>[2x]WGNLGHETVAYIAQSFVASSTESFCQNILGDDSTSYLANVATWADTYKYTDAGEFSKPYHFIDAQDNPPQSCGVDYDRDCGSAGCSISAIQNYTNILLESPNGSEALNALKFVVHIIGDIHQPLHDENLEAGGNGIDVTYDGETTNLHHIWDTNMPEEAAGGYSLSVAKTYADLLTERIKTGTYSSKKDSWTDGIDIKDPVSTSMIWAADANTYVCSTVLDDGLAYINSTDLSGEYYDKSQPVFEELIAKAGYRLAAWLDLIASQPS

S1 nuclease from Aspergillus oryzae (EC 3.1.30.1; NCBI sequence ID: XP_001818636; S1–P1 nuclease family in Pfam, PF02265) is an extracellular, single–strand–specific, sugar non–specific, Zn2+–dependent, fungal nuclease with 3'–mononucleotidase activity with a pH optimum in range 4.0–4.3. S1 nuclease has the phospholipase C/P1 nuclease–like fold stabilized by two disulfide bridges. The active site is located in a surface cleft and composed of the obligatory catalytic trinuclear zinc cluster supplemented by Lys68 and the nucleoside binding site 1 (NBS1; also called Phe site in the previous studies). A cluster of three zinc ions coordinates the substrate/product scissile phosphate and the reaction mechanism utilizes water activated by Zn2+ ions as a nucleophile.

The structure contains two protein chains in the asymmetric unit. Coordination of the zinc ions is completed by four water molecules W1–W4. This structure represents a possible resting state of the enzyme.>GSSLSIRTTDDKSLFARTMDFTMEPDSKVIIVPRNYGIRLL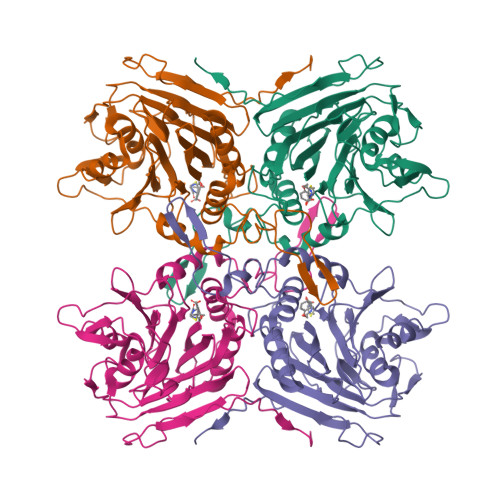EKENVVINNSYAFVGMGSTDITSPVLYDGVNEKGLMGAMLYYATFATYADEPKKGTRGINPVYVISQVLGNCVTVDDVIEKLTSYTLLNEANIILGFAPPLHYTFTDASGESIVIEPDKTGITIHRKTIGVMTNSPGYEWHQTNLRAYIGVTPNPPQDIMMGDLDLTPFGQGAGGLGLPGDFTPSARFLRVAYWKKYTEKAKNETEGVTNLFHILSSVNIPKGVVLTNEGKTDYTIYTSAMCAQSKNYYFKLYDNSRISAVSLMAENLNSQDLITFEWDRKQDIKQLNQVNVMS[2x]4-oxidanylidene-N-[(1S,2R)-2-phenylcyclopropyl]spiro[3H-chromene-2,4'-piperidine]-1'-carboxamide | C23 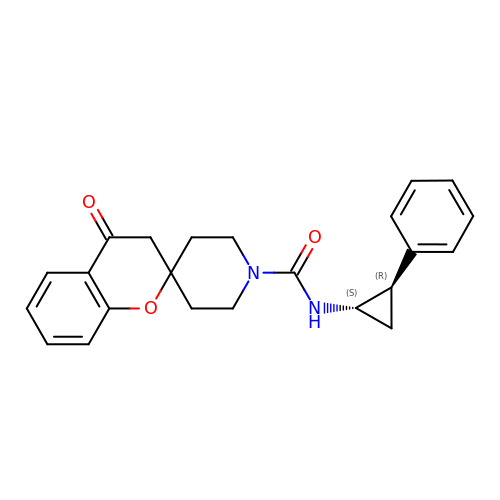H24 N2 O3 | SWEAYHBSAXRXDZ-MOPGFXCFSA-N In response, one family of large bacteriophages uses a nucleus-like compartment to protect its replicating genomes by excluding host defence factors. Here we find that the bacteriophage nuclear shell assembles primarily from one protein, which we name chimallin (ChmA). Combining cryo-electron tomography of nuclear shells in bacteriophage-infected cells and cryo-electron microscopy of a minimal chimallin compartment in vitro, we show that chimallin self-assembles as a flexible sheet into closed micrometre-scale compartments. We find that the shell is primarily composed of a single protein, chimallin, which self-assembles through its extended N and C termini into a closed compartment.

We next purified Goslar chimallin and characterized its self-assembly by SEC–MALS. Similar to 201phi2-1 chimallin, Goslar chimallin forms a mixture of monomers, defined assemblies of around 1.75 MDa, and large aggregates of around 10 MDa. Cryo-EM analysis of the 1.75 MDa assemblies revealed cubic particles approximately 22 nm in diameter, paralleling those formed by 201phi2-1 chimallin. We obtained a 4.2 Å-resolution structure of the overall Goslar chimallin assembly, and used a similar localized reconstruction procedure as for the 201phi2-1 chimallin to obtain a 2.6 Å-resolution structure of the Goslar chimallin tetramer, and a 2.3 Å-resolution structure of a single protomer. The NTS, CTS1 and CTS2 segments of Goslar chimallin show near-identical interactions to neighbouring protomers compared with 201phi2-1 chimallin with the exception of CTS2, which is shorter in Goslar than in 201phi2-1 and shows a distinct set of interactions.

>[24x]SNAMGLDVRNNGNDNVEIRAAETRTAQRADEALETAADFAGQPKVTHTMRTINRTLSRRISRNTGSEQVLNLRRLMEKYLEDTRFKDDFIFVAVDPNQYSVPYPTLVVMSGAKVGDHNHFFGYVLPLVAGLAPLPRREEQGPHGNILVPRTWVDNLNGTFINEVMAAMYAAIGGKSNGTARIAGLAVVTNEITAESAHLATTLLSAADNAIQTAIEIRLGDKLGLPQFNLGMMASDQPISSVQYNTSGMQDSDIVGNPVRSDITVTISNRIRQAMSDYDSQQRLVATTGYIDLTYSPQNPTFNQGPVLVNGYPVPPTVQYQPRYVMTSAYPLELDAFTPNTFVLGLIGTIATLNSGMAWAQSLISNAARGIGPHNPGALAMVLDPEVTAPLDLSTQTNEQIYKFLQQVLYPSLLISIDVPEEGEYSWLLRMIPAAEKIYTGKVEGEVREISEGYKALYRAFDDVTLGCFSKKYQYGLPLVYATGNRIPLGHYNHQDGHRHDIRDMDDLYMMNITNPDTVEAWEDSFDRTDMTMSQRVVARHEIIDRVLSGSWEQTGWAMRYDFDPLALQALIEAAADAGFTIRPENIQHLAGTAVRGNMAARARGLGNISGNIYARSDRPNVGVNNMGGAFNLF>MIPDDEFIKNPSVPGPTAMEVRCLIMCLAEPGKNDVAVDVGCGTGGVTLELAGRVRRVYAIDRNPEAISTTEMNLQRHGLGDNVTLMEGDAPEALCKIPDIDIAVVGGSGGELQEILRIIKDKLKPGGRIIVTAILLETKF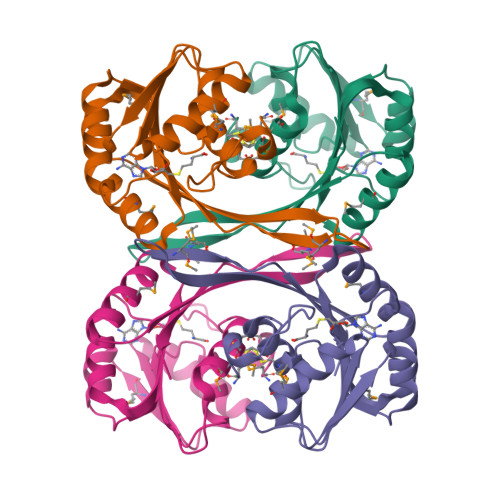EAMECLRDLGFDVNITELNIARGRALDRGTMMVSRNPVALIYTGVSHENKD[6x]> M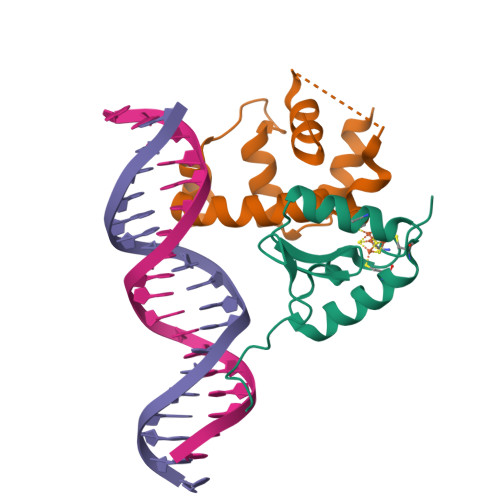SVLTVPRQTPRQRLPVLPCHVGDPDLWFADTPAGLEVAKTLCVSCPIRRQCLAAALQRAEPWGVWGGEIFDQGSIVSHKRPRGRPRKDAVA;> MAHHHHHHVAVDAVSFTLLQDQLQSVLDTLSEREAGVVRLRFGLTDGQPRTLDEIGQVYGVTRERIRQIESKTMSKLRHPSRSQVLRDYLDGSSGSGTPEERLLRAIFGEKA>[2x]GSADK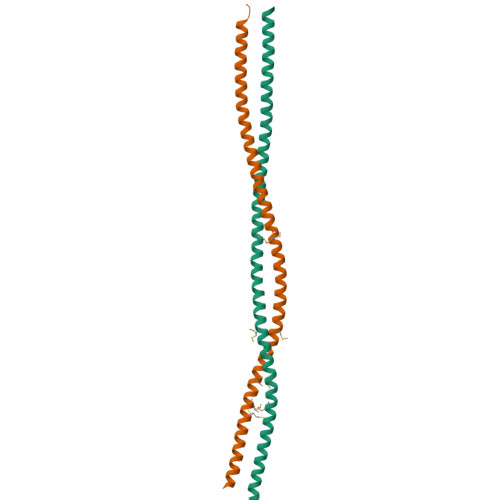SLQESLQKTIYKLEEQLHNEMQLKDEMEQKCRTSNIKLDKIMKELDEEGNQRRNLESTVSQIEKEKMLLQHRINEYQRKAEQENEKRRNVENEVSTLKDQLEDLKKVSQNSQLANEKLSQLQKQLEEA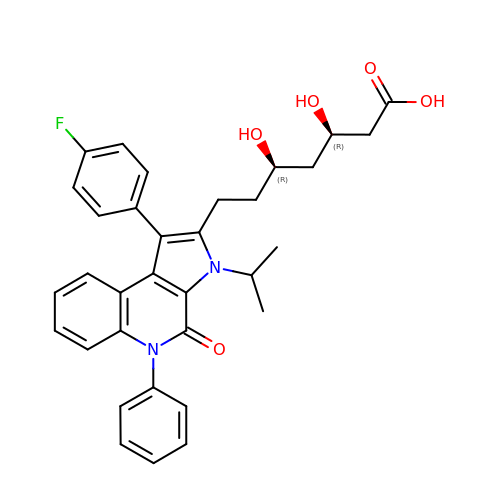(3R,5R)-7-[1-(4-FLUOROPHENYL)-3-ISOPROPYL-4-OXO-5-PHENYL-4,5-DIHYDRO-3H-PYRROLO[2,3-C]QUINOLIN-2-YL]-3,5-DIHYDROXYHEPTANOIC ACID | C33 H33 F N2 O5 | UFHOPRVARZPTSH-JWQCQUIFSA-N> MGTSLT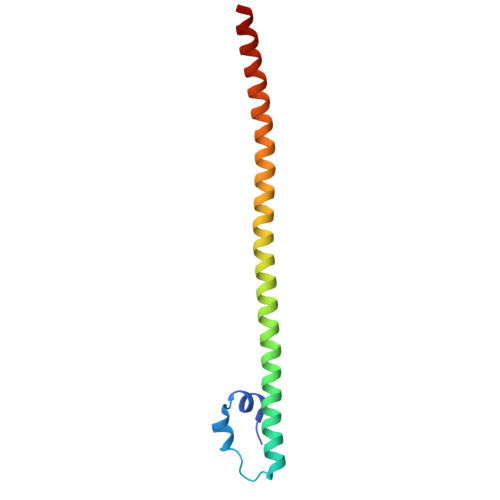DEELVTMSVRELNQHLRGLSKEEIVQLKQRRRTLKNRGYAASCRVKRVTQKEELEKQKAELQQEVEKLASENASMKLELDALRSKYEALQTFARTVAR Cedar virus (CedV) is a Henipavirus species isolated from the excreta of Pteropus bat colonies in Queensland, Australia. HNV-G proteins comprise a short N-terminal cytosolic region, single-pass transmembrane domain, oligomerization-mediating and fusion-activating stalk region, and C-terminal receptor-binding β-propeller domain. Binding of the HNV-G to cell surface receptors belonging to the ephrin ligand family initiates pH-independent activation of F, triggering a fusion cascade that results in the ultimate merger of viral and cellular membranes. In our integrated structural and functional analysis, we demonstrate that in addition to using the common HNV receptor, ephrin-B2, CedV uses ephrin-B1, a receptor with no precedent of HNV usage.

To this end, we solved the crystal structure of the attachment-mediating β-propeller of CedV-G in complex with the extracellular β-barrel domain of human ephrin-B1, to 4.07-Å resolution. Five complexes populated the crystallographic a.s.u. and displayed no appreciable structural variation, within the limits of the resolution. Comparison with the unliganded structure of CedV-G reveals little overall structural variation (0.4 Å RMSD over 417 equivalent Cα) within the ephrin-B1–bound CedV-G scaffold. CedV-G engages ephrin-B1 with an overall binding mode that is similar to that used by other HNV-G proteins, when recognizing their respective ephrin receptors. CedV-G and ephrin-B1 form a 1:1 complex with an extensive molecular interface that buries a combined surface area of 2,900 Å2 (1,450 Å2 per component). Ephrin-B1 is bound at the top of the molecule and forms an interface that chiefly comprises residues from the structurally conserved β4–6 blades of CedV-G, which contribute ∼70% (∼2,000 Å2) of the total buried surface area. Like the other HNV-G–ephrin complexes, the G–H loop of ephrin-B1 (residues 113–129ephrin−B1) constitutes a major interacting region and is inserted into the central depression on top of CedV-G, contributing 1,700-Å2 buried surface area to the molecular interface. Inspection of the CedV-G–ephrin-B1 complex structure reveals that the side chain of Tyr121−ephrin-B1 is inserted into a large hydrophobic cavity that is unique to CedV-G. Indeed, the equivalent region within NiV-G (Trp504), HeV-G (Trp504), and GhV-G (Trp514) is, in all instances, occluded by a tryptophan side chain that protrudes toward the toroidal axis of the β-propeller, rather than being sequestered in the opposing direction as is the equivalent residue, Tyr525−CedV-G. Thus, it is likely that the expanded hydrophobic cavity of CedV-G is critical to ephrin-B1 recognition as it circumvents steric clashes that would preclude its recognition by other HNV-Gs.

>ETGKIFCKSVSKDPDFRLKQIDYVIPVQQDRSICMNNPLLDISDGFFTYIHYEGINSCKKSDSFKVLLSHGEIVDRGDYRPSLYLLSSHYHPYSMQVINCVPVTCNQSSFVFCHISNNTKTLDNSDYSSDEYYITYFNGIDRPKTKKIPINNMTADNRYIHFTFSGGGGVCLGEEFIIPVTTVINTDVFTHDYCESFNCSVQTGKSLKEICSESLRSPTNSSRYNLNGIMIISQNNMTDFKIQLNGITYNKLSFGSPGRLSKTLGQVLYYQSSMSWDTYLKAGFVEKWKPFTPNWMNNTVISRPNQGNCPRYHKCPEICYGGTYNDIAPLDLGKDMYVSVILDSDQLAENPEITVFNSTTILYKERVSKDELNTRSTTTSCFLFLDEPWCISVLETNRFNGKSIRPEIYSYKIPKYCGTKHHHHHH[5x];>[5x]ETGAKNLEPVSWSSLNPKFLSGKGLVIYPKIGDKLDIICPRAEAGRPYEYYKLYLVRPEQAAACSTVLDPNVLVTCNRPEQEIRFTIKFQEFSPNYMGLEFKKHHDYYITSTSNGSLEGLENREGGVCRTRTMKIIMKVGQDGTKHHHHHH>[5x]MDYLFKLLLIGDSGVGKTCVLFRFSEDAFNSTFISTIGIDFKIRTIELDGKRIKLQIWDTAGQERFRTITTAYYRGAMGIMLVYDITNEKSFDNIRNWIRNIEEHASADVEKMILGNKCDVNDKRQVSKERGEKLALDYGIKFMETSAKANINVENAFFTLARDIKAKMDKKHHHHHH

Upon attachment to their target membranes, Rab GTPases act as molecular switches that are activated by a GEF that catalyzes the exchange of the bound guanosine-5′-diphosphate (GDP) for the more abundant guanosine-5′-triphosphate (GTP). Once active, the GTP-bound Rab can interact with specific effector proteins which mediate a variety of downstream functions including binding to cargoes, enabling vesicle formation and promoting vesicle fusion to target membranes. Rabs are inactivated by GAPs that promote the hydrolysis of GTP to GDP and the inactive Rab is then relocalized to the cytosol. Structural analysis of Rab8A revealed that the PINK1-regulated Ser111 site lies within a short stretch of amino acids within the C-terminal region termed the RabSF3 motif (see Supplementary Figure S3 for a structural depiction of Rab regions and position of Ser111 and Thr72 residues).

To understand the mechanism by which Ser111 phosphorylation impacts on its interactions with its GEF, GAP and LRRK2, we solved the structure of pSer111-Rab8A. Phosphorylated Rab8A exhibits a typical small GTPase fold with highly flexible Switch regions in the GDP-bound form, and well-defined structured Switch regions in the GppNHp-bound form. The pSer111 residue is located C-terminal of helix α3 in a loop above the Switch II region (α2). The superimposed structures of pSer111-Rab8A and WT-Rab8A showed that the phosphorylation at Ser111 does not impact the overall structure of Rab8A. Interestingly, the formation of a new intramolecular interaction between the phosphate group and the side chain of Arg79 at the C-terminal end of Switch II is striking in the structure of pSer111-Rab8A:GDP. Consistent with this possibility, the Rab8A:Rabin8 structure has recently been analyzed using molecular dynamics simulation revealing a salt-bridge interaction between residue Asp187 of Rabin8 with Arg79 that lies within the Switch II domain of Rab8A. This is consistent with the observation that an intramolecular H-bond is created by the presence of the phosphate at Ser111 with the side chain of Arg79. Ser111 is located opposite a negative surface patch of Rabin8 in proximity to Asp187. Thus addition of a negative charge at Ser111 either by S111E or pSer111 disrupts the interaction between Asp187 of Rabin8 and Arg79 of the Rab8A. Strikingly, we found that the ability of LRRK2 [G2019S] to phosphorylate pSer111-Rab8A:GDP was disrupted (compared with WT-Rab8A:GDP) and a similar reduction was determined for pSer111-Rab8A:GppNHp (compared with WT-Rab8A:GppNHp).>[2x]MPGLFLTLEGLDGSGKTTQARRLAAFLEAQGRPVLLTREPGGGLPEVRSLLLTQELSPEAEYLLFSADRAEHVRKVILPGLAAGKVVISLRYLDSS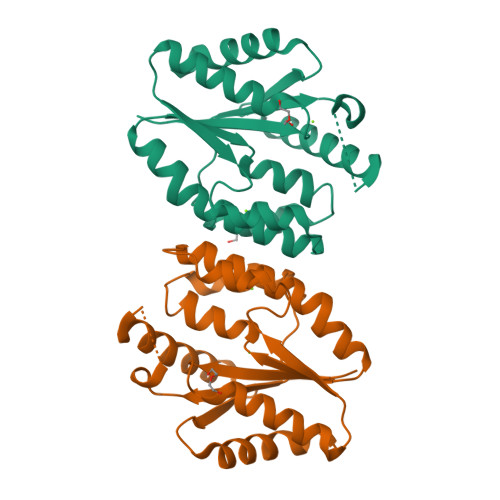LAYQGYGRGLPLPWLREVAREATRGLKPRLTFLLDLPPEAALRRVRRPDRLEGLGLEFFRRVREGYLALARAEPGRFVVLDATLPEEEIARAIQAHLRPLLP> TMGGDALRVPFLDFATATPKRHQTVVPGVGTLHDCCEHSPLFSAVARRLLFNSLVPAQLKGRDFGGDHTAKLEFLAPELVRAVARLRFKECAPADVVPQRNAYYSVLNTFQALHRSEAFRQLVHFVRDFAQLLKTSFRASSLTETTGPPKKRAKVDVATHGRTYGTLELFQKMILMHATYFLAAVLLGDHAEQVNTFLRLVFEIPLFSDAAVRHFRQRATVFLVPRRHGKTWFLVPLIALSLASFRGIKIGYTAHIRKATEPVFEEIDACLRGWFGSARVDHVKGETISFSFPDGSRSTIVFASSHNTNGIRGQDFNLLFVDEANFIRPDAVQTIMGFLNQANCKIIFVSSTNTGKASTSFLYNLRGAADELLNVVTYICDDHMPRVVTHTNATACSCYILNKPVFITMDGAVRRTADLFLADSFMQEIIGGQARETGDDRPVLTKSAGERFLLYRPSTTTNSGLMAPDLYVYVDPAFTANTRASGTGVAVVGRYRDDYIIFALEHFFLRALTGSAPADIARCVVHSLTQVLALHPGAFRGVRVAVEGNSSQDSAVAIATHVHTEMHRLLASEGADAGSGPELLFYHCEPPGSAVLYPFFLLNKQKTPAFEHFIKKFNSGGVMASQEIVSATVRLQTDPVEYLLEQLNNLTETVSPNTDVRTYSGKRNGASDDLMVAVIMAIYLAAQAGPPHT;> AAPVSEPTVARQKLLALLGQVQTYVFQIELLRRCDPHIGRGKLPQLKLNALQVRALRRRLRPGLEAQAGAFLTPLSVTLELLLEYAWREGERLLGSLETFATAGDVAAFFTETMGLARPCPYHQRVRLDTYGGTVHMELCFLHDVENFLKQLNYCHLITPSRGATAALERVREFMVGAVGSGLIVPPELSDPSHPCAVCFEELCVTANQGATIASRLADRICNHVTQQAQVRLDANELRRYLPHAAGLSDADRARALSVLDHALARTAGGDGQPHPSPENDSVRKEADALLEAHDVFQATTPGLYAISELQFWLASGDRAGQTTMDAFASNLTALARRELQQETAAVAVELALFGRRAEHFDRAFGSHLAALDMVDALIIGGQATSPDDQIEALIRACYDHHLTTPLLRRLVSPEQCDEEALRRVLARMGAGGAADAPKGGAGPDDDGDRVAVEEGARGLGAPGGGGEDEDRRRGPGGQGPETWGDIATQAAADVRERRRLYADRLTKRSLASLGRCVREQRGELEKMLRVSVHGEVLPATFAAVANGFAARARFCALTAGAGTVIDNRSAPGVFDAHRFMRASLLRHQVDPALLPSITHRFFELVN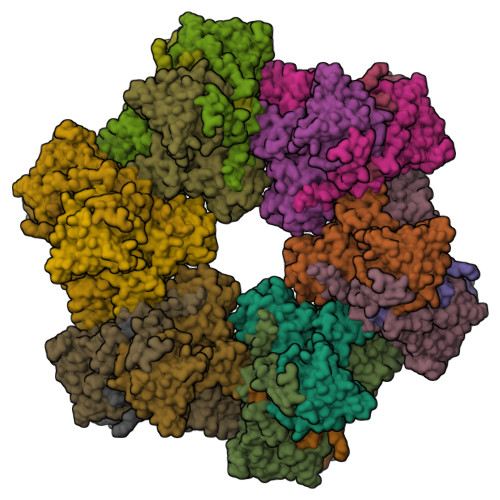GPLFDHSTHSFAQPPNTALYYSVENVGLLPHLKEELARFIMGAGGSGADWAVSEFQRFYCFDGISGITPTQRAAWRYIRELIIATTLFASVYRCGELELRRPDCSRPTSEGRYRYPPGVYLTYDSDCPLVAIVESAPDGCIGPRSVVVYDRDVFSILYSVLQHLAPR;> TLRDTIPDCALRSQTLESLDARYVSRDGAHDAAVWFEDMTPAELEVVFPTTDAKLNYLSRTQRLASLLTYAGPIKAPDDAAAPQTPDTACVHGELLARKRERFAAVINRFLDLHQILR>[4x]SNAMRKDETSNTSPDISVAQPASALRYHLRPPRRNDGAAIHQLVSECPPLDL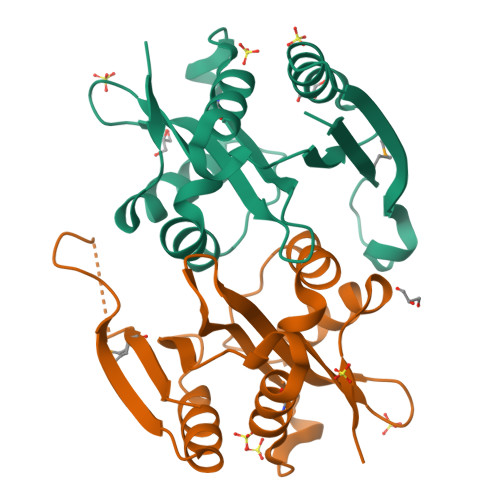NSLYAYLLLCEHHAHTCVVAESPGGRIDGFVSAYLLPTRPDVLFVWQVAVHSRARGHRLGRAMLGHILERQECRHVRHLETTVGPDNQASRRTFAGLAGERGAHVSEQPFFDRQAFGGADHDDEMLLRIGPFTHPPH> GSMRAHLLDNTERLERSSRRLEAGYQIAVETEQIGQEMLENLSHDRERIQRARERLRETDANLGKSSRI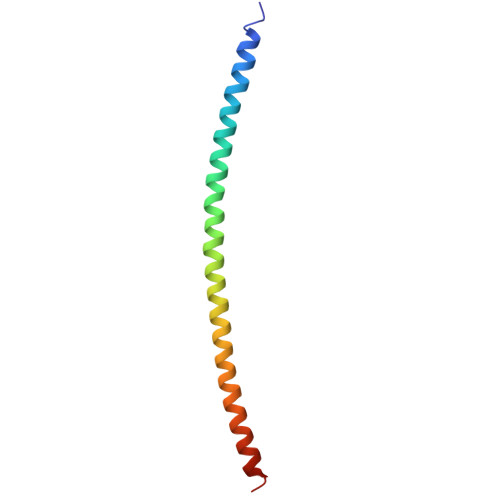LTGMLRRIIQNR>MGSSHHHHHHSSGLVPRGSSDRPEDAIAIVGMSGRYPGARNVREYWDNLVHARNAIRDIPTSRWDVDKYYDPVLNKKGKVYCKSMGMLDDIEHFDPLFFNIPPSEAELMDPQHRIFLQEGYKAFEDAGYNARTLNEKKCGVYLGIMSNEYGVMLNRQSRANATGNSFAIAAARIPYFLNLKGPAIPIDTACSSSLVGTHLARQALINKEIDMALVGGVSLYLTPESYMSMCEAGMLSPDGQCKAFDNGANGFVPGEGAGALVLKRLKDAEADRDHIYGIIIGSGINQDGKTNGITAPSAKSQMDLERDIYETYGIHPESISYVEMHGTGTKQGDPIELEALSTVFQEKTDKKQFCAIGSVKSNIGHTSAAA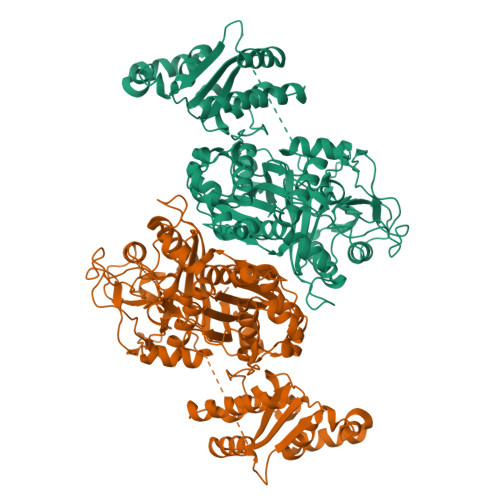GVAGVQKVLLCMNHKTLVPTLNFTTPNEHFEFEHSPLYVNTELKPWETADGKPRRACVSSFGYSGTNAHIVIEEYQPEKRNDRLTKQHRSALFVLSAKKEKQLKAYAEAMKDFVTSNEDIDLEDMAYTLQTGREAMDYRMAFLADSREMLIKALDDYLAEMPNGSIFAAHVKTKKSEIKLFETDHDAKALLQTWIEKKRLEKVAELWVKGLQIDWNKLYGEYTPRRISLPAYPFAEEYYWLPTQEG[2x]>GCAG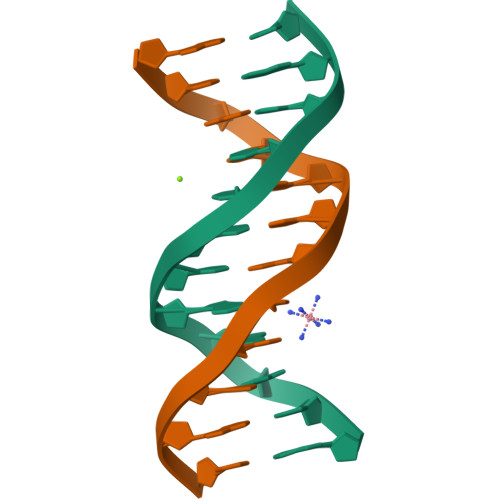ACGTCTGC[6x]> GSGTMQTFLKGKRVGYWLSEKKIKKLNFQAFAELCRKRGMEVVQLNLSRPIEEQGPLDVIIHKLTDVILEADQNDSQSLELVHRFQEYIDAHPETIVLDPLPAIRTLLDRSKSYELIRKIEAYMEDDRICSPPFME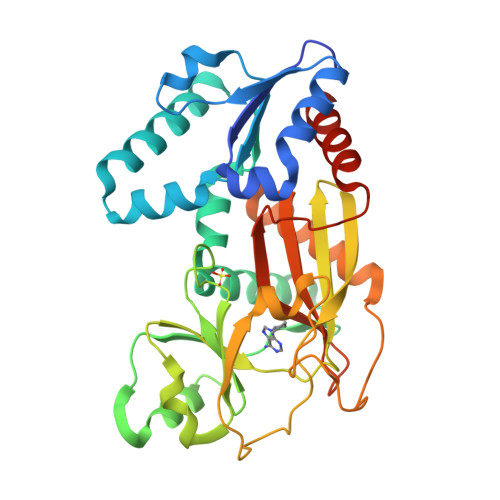LTSLCGDDTMRLLEKNGLTFPFICKTRVAHGTNSHEMAIVFNQEGLNAIQPPCVVQNFINHNAVLYKVFVVGESYTVVQRPSLKNFSAGTSDRESIFFNSHNVSKPESSSVLTELDKIEGVFERPSDEVIRELSRALRQALGVSLFGIDIIINNQTGQHAVIDINAFPGYEGVSEFFTDLLNHIATVLQGQSTAM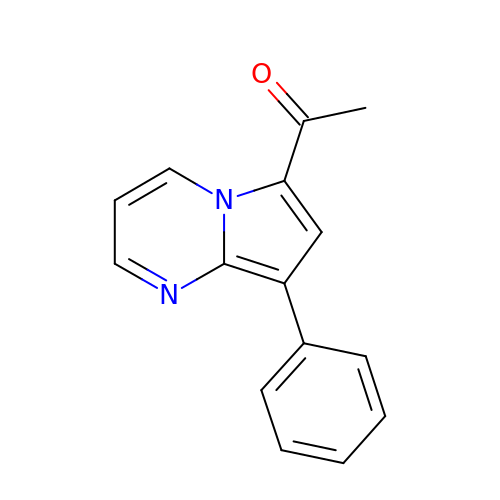1-(8-phenylpyrrolo[1,2-a]pyrimidin-6-yl)ethanone | C15 H12 N2 O | FPBCLTMMKANZAZ-UHFFFAOYSA-N>MYRTHYSSEITEELNGQKVKVAGWVWEVKDLGGIKFLWIRDRDGIVQITAPKKKVDPELFKLIPKLRSEDVVAVEGVVNFTPKAKLGFEILPEKIVVLNRAETPLPLDPTGKVKAE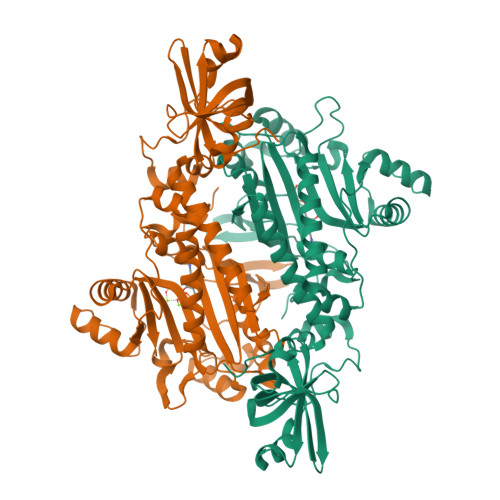LDTRLDNRFMDLRRPEVMAIFKIRSSVFKAVRDFFHENGFIEIHTPKIIATATEGGTELFPMKYFEEDAFLAQSPQLYKQIMMASGLDRVYEIAPIFRAEEHNTTRHLNEAWSIDSEMAFIEDEEEVMSFLERLVAHAINYVREHNAKELDILNFELEEPKLPFPRVSYDKALEILGDLGKEIPWGEDIDTEGERLLGKYMMENENAPLYFLYQYPSEAKPFYIMKYDNKPEICRAFDLEYRGVEISSGGQREHRHDILVEQIKEKGLNPESFEFYLKAFRYGMPPHGGFGLGAERLIKQMLDLPNIREVILFPRDRRRLTP[2x]> MHRSTGIGVSRWLGGLLGVALALPALALPQGCIELLAQAPRVDVVQGQQRDLRLAVPIERLAIGDPKIADVQLLDRRGFLVTGKEQGSTSLLIWTGCSPEPLRSLVEVEGRGSVDTRGAPAFTVGAAEELPNQVQTDIRFVEVSRSKLKQASTSFVRRGGNLWVLGAPGSLGDIKVNADGSGLGGTFGTGSSGFNLIFGGGKWLSFMNAL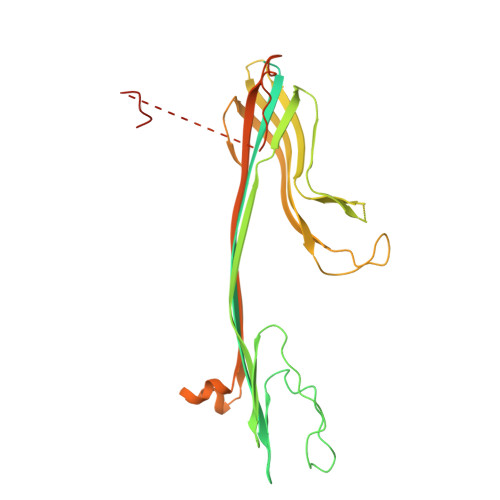EGSGFAYTLARPSLVAMSGQSASFLAGGEFPIPVPNGTNDNVTIEYKEFGIRLTLTPTVMNNRRIALKVAPEVSELDYSAGIQSGGVAVPALRVRRTDTSVMLADGESFVISGLTSSNSVSNVDKFPWLGDIPILGAFFRSTKLDKDDRELLMIVTPHLVQPLAADAQLPDLPGEGLRHYDPGFSRLYFLERGEYDGQQNDTGLSDSAWSHPQFEK>[2x]MLFYSFFKTLIDTEVTVELKNDMSIRGILKSVDQFLNVKL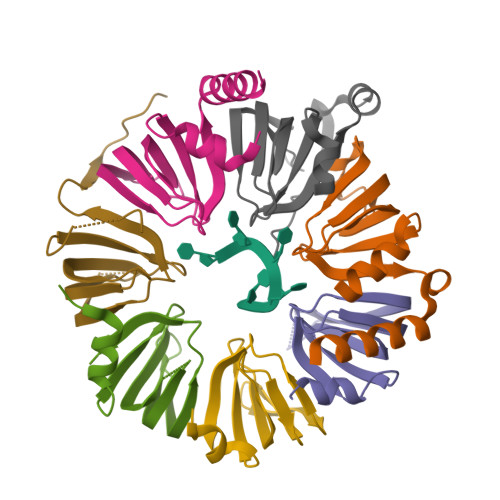ENISVVDASKYPHMAAVKDLFIRGSVVRYVHMSSAYVDTILLADACRRDLANNKRQ;>[2x]GSMESAQAVAEPLDLVRLSLDEIVYVKLRGDRELNGRLHAYDEHLNMVLGDAEEIVTIFDDEETDKDKALKTIRKHYEMLFVRGDSVILIAPPRN;>[2x]MLPLTLLNATQGRPILVELKNGETFNGHLENCDNYMNLTLREVIRTMPDGDKFFRLPECYIRGNNIKYLRIQDEVLSQVAKQQAQQRENRGSRFRGRGQRGRGNYGHTAPNRRGRGRGGHMWSHPQFEK;>[2x]MSMTILPLELIDKCIGSNLWVIMKSEREFAGTLVGFDDYVNIVLKDVTEYDTVTGVTEKHSEMLLNGNGMCMLIPGGKPE;>[2x]GSMDSSPNEFLNKVIGKKVLIRLSSGVDYKGILSCLDGYMNLALERTEEYVNGKKTNVYGDAFIRGNNVLYVSALDD;>[2x]MSSLQKRPGPGNSSQPTERPRKESILDLSRYQDQRIQATFTGGRQITGILKGFDQLMNLVLDDVEEQLRNPEDGKLTGAIRKLGLVVVRGTTLVLIAPMDGSEEIPNPFVQAEHHHHHH;>MSLADFMEQRVQVITNDGRVVLGSLKGFDHTTNLILSDSFERIISMDQDMETIPLGVYLLRGENVAMVGLVNEELDSEIEWTKIRGEAIPDVVH[2x]>[4x]MGSSHHHHHHSSGRENLYFQGMKETNSEEADSGLAFFRNMYDKYRDAFLSHLNEYSLEEEIKEHISKYYKLLFDYNCLGGKNNRGILVILIYEYVKNRDINSSEWEKAACLAWCIE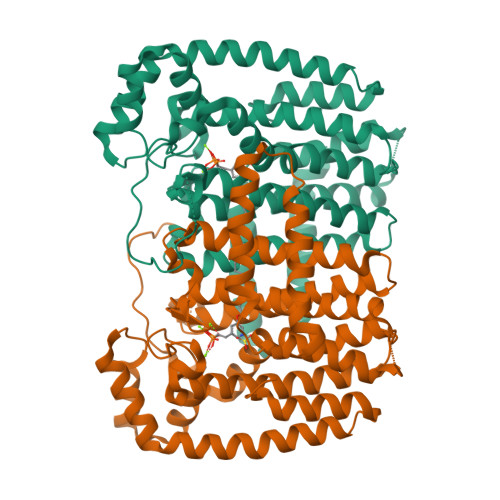ILQAAFLVADDIMDKGEMRRNKYCWYLLKDVETKNAVNDVLLLYNSIYKLIEIYLRNESCYVDVIATFRDATLKTIIGQHLDTNIFSDKYSDAHREIDVNNINVPEQPVIDINMINFGVYKNIVIHKTAYYSFFLPIVCGMLLAGIAVDNLIYKKIEDISMLMGEYFQIHDDYLDIFGDSTKTGKVGSDIQNNKLTWPLIKTFELCSEPDKIKIVKNYGKNNLACVKVIDSLYEQYKIRKHYESYEKAQKAKILSAINELHHEGIEYVLKYLLEILFTGV> MKKEKIDLFYGALLHDIGKVIQRATGERKKHALVGADWFDEIADNQVISDQIRYHMANYQSDKLGNDHLAYITYIADNIASGVDRRQSNEESDEDASAKIWDTYTNQADIFNVFGAQTDKRYFKPTVLNLKSKPNFASATYEPFSKGDYAAIATRIKNELAEFEFNQAQIDSLLNLFEAILSFVPSSTNSKEIADISLAEHSRLTAAFALAIYDYLEDKGRHNYKEDLFTKASAFYEEEAFLLASFDLSGIQDFIYNIATSGAAKQLKARSLYLDFMSEYIADSLLDKLGLNRANLLYVGGGHAYFVLANTEKTVETLVQFEKDFNQFLLANFQTRLYVAFGWGSFAAKDIMSELNSPESYRQIYQKASRMISEKKISRYDYRTLMLLNRGGKSSERECEICHSVENLVSYHDQKVCDICRGLYQFSKEIAHDHFIITENEGLPIGPNACLKGVAFEKLSQESFSRVYVKNDYKAGTIKATHVFVGDYQCDEIHKYAALSKNEDGLGIKRLAVVRLDVDDLGAAFMAGFSRQGNGQYSTLSRSATFSRSMSLFFKVYINQFASDKKLSIIYAGGDDVFAIGSWQDIIAFTVELRQNFIKWTNGKLTLSAGIGLFADKTPISLMAHQTGELEEAAKGNEKDSISLFSSDY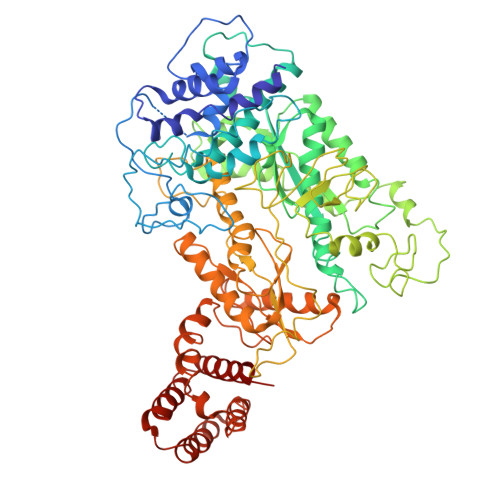TFKFDRFITNVYDDKLEQIRYFFNHQDERGKNFIYKLIELLRNYESEEKMNVARLAYYLTRLEELTDKDERDKFKQFKKLFFKWYTNNESDRKEAELALLLYVYEIRKD> MSLISKEELIKLAYSIRPRENEYKTILTNLDEYNKLTTNNNENKYLQLKKLNESIDVFMNKYKNSSRNRALSNLKKDILKEVILIKNSNTSPVEKNLHFVWIGGEVSDIALEYIKQWADINAEYNIKLWYDSEAFLVNTLKKAIVESSTTEALQLLEEEIQNPQFDNMKFYKKRMEFIYDRQKRFINYYKSQINKPTVPTIDDIIKSHLVSEYNRDETLLESYRTNSLRKINSNHGIDIRANSLFTEQELLNIYSQELLNRGNLAAASDIVRLLALKNFGGVYLDVDMLPGIHSDLFKTIPRPSSIGLDRWEMIKLEAIMKYKKYINNYTSENFDKLDQQLKDNFKLIIESKSEKSEIFSKLENLNVSDLEIKIAFALGSVINQALISKQGSYLTNLVIEQVKNRYQFLNQHLNPAIESDNNFTDTTKIFHDSLFNSATAENSMFLTKIAPYLQVGFMPEARSTISLSGPGAYASAYYDFINLQENTIEKTLKASDLIEFKFPENNLSQLTEQEINSLWSFDQASAKYQFEKYVRDYTGGSLSEDNGVDFNKNTALDKNYLLNNKIPSNNVEEAGSKNYVHYIIQLQGDDISYEATCNLFSKNPKNSIIIQRNMNESAKSYFLSDDGESILELNKYRIPERLKNKEKVKVTFIGHGKDEFNTSEFARLSVDSLSNEISSFLDTIKLDISPKNVEVNLLGCNMFSYDFNVEETYPGKLLLSIMDKITSTLPDVNKDSITIGANQYEVRINSEGRKELLAHSGKWINKEEAIMSDLSSKEYIFFDSIDNKLKAKSKNIPGLASISEDIKTLLLDASVSPDTKFILNNLKLNIESSIGDYIYYEKLEPVKNIIHNSIDDLIDEFNLLENVSDELYELKKLNNLDEKYLISFEDISKNNSTYSVRFINKSNGESVYVETEKEIFSKYSEHITKEISTIKNSIITDVNGNLLDNIQLDHTSQVNTLNAAFFIQSLIDYSSNKDVLNDLSTSVKVQLYAQLFSTGLNTIYDSIQLVNLISNAVNDTINVLPTITEGIPIVSTILDGINLGAAIKELLDEHDPLLKKELEAKVGVLAINMSLSIAATVASIVGIGAEVTIFLLPIAGISAGIPSLVNNELILHDKATSVVNYFNHLSESKEYGPLKTEDDKILVPIDDLVISEIDFNNNSIKLGTCNILAMEGGSGHTVTGNIDHFFSSPYISSHIPSLSVYSAIGIKTENLDFSKKIMMLPNAPSRVFWWETGAVPGLRSLENNGTKLLDSIRDLYPGKFYWRFYAFFDYAITTLKPVYEDTNTKIKLDKDTRNFIMPTITTDEIRNKLSYSFDGAGGTYSLLLSSYPISMNINLSKDDLWIFNIDNEVREISIENGTIKKGNLIEDVLSKIDINKNKLIIGNQTIDFSGDIDNKDRYIFLTCELDDKISLIIEINLVAKSYSLLLSGDKNYLISNLSNTIEKINTLGLDSKNIAYNYTDESNNKYFGAISKTSQKSIIHYKKDSKNILEFYNGSTLEFNSKDFIAEDINVFMKDDINTITGKYYVDNNTDKSIDFSISLVSKNQVKVNGLYLNESVYSSYLDFVKNSDGHHNTSNFMNLFLNNISFWKLFGFENINFVIDKYFTLVGKTNLGYVEFICDNNKNIDIYFGEWKTSSSKSTIFSGNGRNVVVEPIYNPDTGEDISTSLDFSYEPLYGIDRYINKVLIAPDLYTSLININTNYYSNEYYPEIIVLNPNTFHKKVNINLDSSSFEYKWSTEGSDFILVRYLEESNKKILQKIRIKGILSNTQSFNKMSIDFKDIKKLSLGYIMSNFKSFNSENELDRDHLGFKIIDNKTYYYDEDSKLVKGLININNSLFYFDPIESNLVTGWQTINGKKYYFDINTGAASTSYKIINGKHFYFNNNGVMQLGVFKGPDGFEYFAPANTQNNNIEGQAIVYQSKFLTLNGKKYYFDNDSKAVTGWRIINNEKYYFNPNNAIAAVGLQVIDNNKYYFNPDTAIISKGWQTVNGSRYYFDTDTAIAF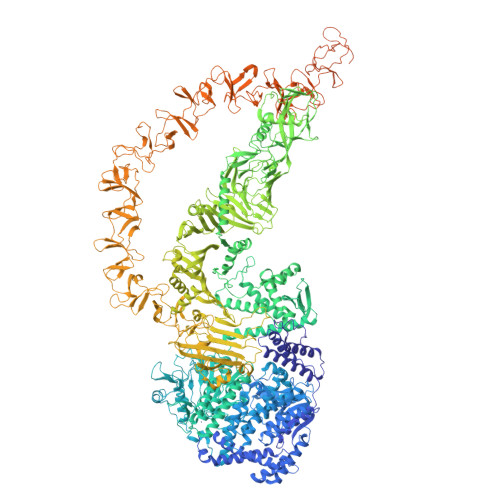NGYKTIDGKHFYFDSDCVVKIGVFSGSNGFEYFAPANTYNNNIEGQAIVYQSKFLTLNGKKYYFDNNSKAVTGWQTIDSKKYYFNTNTAEAATGWQTIDGKKYYFNTNTAEAATGWQTIDGKKYYFNTNTSIASTGYTIINGKYFYFNTDGIMQIGVFKVPNGFEYFAPANTHNNNIEGQAILYQNKFLTLNGKKYYFGSDSKAITGWQTIDGKKYYFNPNNAIAATHLCTINNDKYYFSYDGILQNGYITIERNNFYFDANNESKMVTGVFKGPNGFEYFAPANTHNNNIEGQAIVYQNKFLTLNGKKYYFDNDSKAVTGWQTIDSKKYYFNLNTAVAVTGWQTIDGEKYYFNLNTAEAATGWQTIDGKRYYFNTNTYIASTGYTIINGKHFYFNTDGIMQIGVFKGPDGFEYFAPANTHNNNIEGQAILYQNKFLTLNGKKYYFGSDSKAVTGLRTIDGKKYYFNTNTAVAVTGWQTINGKKYYFNTNTYIASTGYTIISGKHFYFNTDGIMQIGVFKGPDGFEYFAPANTDANNIEGQAIRYQNRFLYLHDNIYYFGNDSKAATGWATIDGNRYYFEPNTAMGANGYKTIDNKNFYFRNGLPQIGVFKGPNGFEYFAPANTDANNIDGQAIRYQNRFLHLLGKIYYFGNNSKAVTGWQTINSKVYYFMPDTAMAAAGGLFEIDGVIYFFGVDGVKAPGIYG> SNAMSDLVSYHLDDGVATLTLNNGKVNAISPDVIIAFNAALDQAEKDR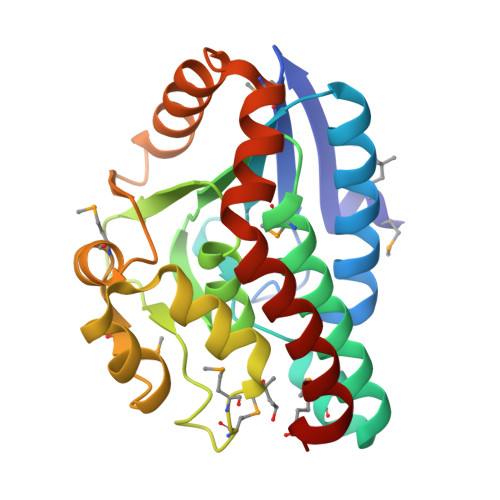AIVIVTGQPGILSGGYDLKVMTSSAEAAINLVAQGSTLARRMLSHPFPIIVACPGHAVAKGAFLLLSADYRIGVAGPFSIGLNEVQIGMTMHHAGIELARDRLRKSAFNRSVINAEMFDPEGAMAAGFLDKVVSVEELQGAALAVAAQLKKINMNAHKKTKLKVRKGLLDTLDAAIEQDRQHML>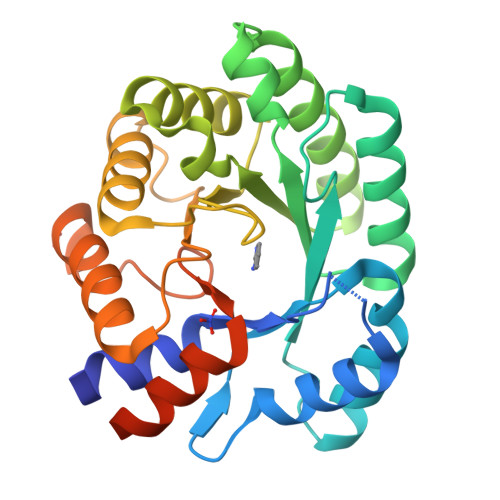 MATDLKASSLRALKLMHLATSANDDDTDENVIALCHQAKTPVGTTDAIFIYPRFIPIARKTLKEQGTPEIRICTSTNFPHGNDDIDIALAETRAAIAYGADGVAVVFPYRALMAGNEQVGFDLVKACKEACAAANVLLSVIIETGELKDEALIRKASEISIKAGADYIVTSTGKVAVGATPESARIMMEVIRDMGVENTVGFIPVGGVRTAEDAQKYLAIADELFGADWADARHYAFGASGSLLASLLKALGHGDGKSASSYGSLEHHH>[4x]GPLGSKEQGVVRKAGWLFFKPLVTLQKERKLELVARRKWKQYWVTLKGCTLLFYETYG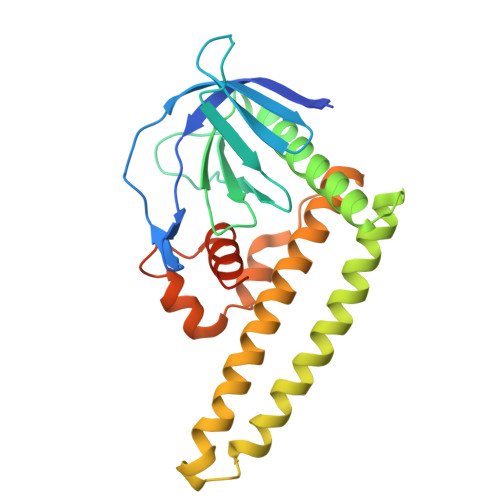KNSTEQNSAPRCALFAEDSIVQSVPEHPKKEHVFCLSNSCGDVYLFQATSQTDLENWVTAIHSACASLFAKKHGKEDTVRLLKSQTRSLLQKIDMDSKMKKMAELQLSVVSDPKNRKAIENQIRQWEQNLEKFHMDLFRMRCYLASLQGGELPNPKSLLAATSRPSKLALGRLGVLSVSSFHALVCSRDDSTLRKRTLSLTQRGK(2~{S})-4-methyl-2-[[(2~{S})-3-oxidanyl-2-[[oxidanyl(phenylmethoxycarbonylaminomethyl)phosphoryl]amino]propanoyl]amino]pentanoic 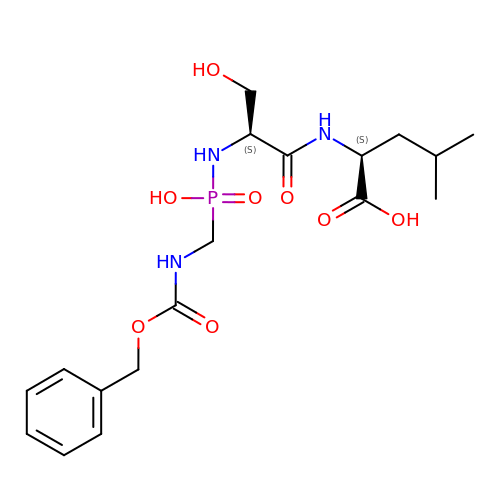acid | C18 H28 N3 O8 P | SSYZVHUEGYLORV-GJZGRUSLSA-N> EE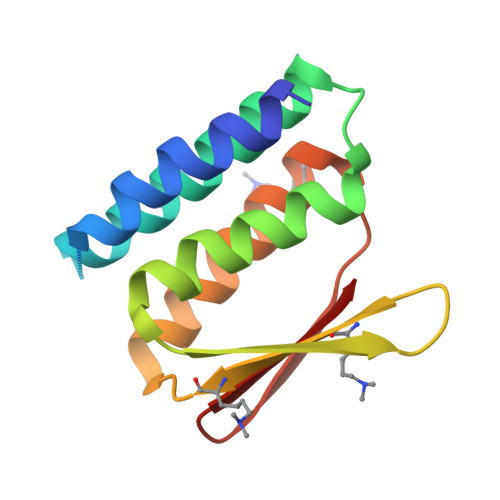AVRRRFEELLREALAFRERTGGRRETLEHAVRLARELAEFAASHPEFNRQEAVLLAIELMVRAMGVTMETHRSGNEVKVVIKGLNIDEQVALYRAVRETSKIMGVETEIEVEGDTQTIVV Cyclic GMP‐AMP synthase (cGAS)* is a sensor of cytosolic double‐stranded DNA (ds‐DNA). ds‐DNA in the cytosol may occur from infection or mitochondrial damage. cGAS is activated by ds‐DNA binding to catalyze the cyclization of ATP and GTP to form a cyclic dinucleotide with mixed 2′,5′‐ and 3′,5′‐phosphodiester linkage (2′,3′‐cGAMP), which in turn activates stimulator of type 1 interferon genes (STING). Activated STING causes the activation of TBK1, which phosphorylates IRF3 allowing it to translocate to the nucleus where it triggers interferon‐inducible gene activation and interferon production. We report here the structure of cGAS with dinucleotides and small molecule inhibitors, and kinetic studies of the cGAS mechanism.

To study the β‐pseudo‐active form we obtained structures of an N‐terminal truncation of cGAS starting at residue 161 (cGAS161)22 in complex with five cyclic dinucleotides (2′,2′‐cGAMP, 2′,3′‐cGAMP, 3′,3′‐cGAMP, 3′,3′‐cdIMP and 3′,3′‐cdUMP), and the linear 2′,5′‐GpAp dinucleotide. There is no interaction between Asp227 and 3′,3′‐cdUMP or 2′,2′‐cGAMP; in these structures cGAS retains an inactive pose. 2′,2′‐cGAMP contains an amino group on its guanine base; however, 2′,2′‐cGAMP is considerably displaced from the active site compared with 2′,3′‐cGAMP or 3′,3′‐cGAMP with its amino group interacting with Asp319 (2.9 Å) instead of Asp227. Each compound binds to the same site formed between the side chains of Tyr436 and Arg376. This site is occupied by the adenine base in structures of ATP, 2′,2′‐cGAMP, 2′,3′‐cGAMP, or 3′,3′‐cGAMP, and is composed primarily of London dispersion interactions between the ring system of these binders with the phenyl ring of Try436. Most of these dinucleotides have affinities weaker than 500 μM (the top concentration tested).

>[2x]MGASKLRAVLEKLKLSRDDISTAAGMVKGVVDHLLLRLKCDSAFRGVGLLNTGSYYEHVKISAPNEFDVMFKLEVPRIQLEEYSNTRAYYFVKFKRNPKENPLSQFLEGEILSASKMLSKFRKIIKEEINDIKDTDVIMKRKRGGSPAVTLLISEKISVDITLALESKSSWPASTQEGLRIQNWLSAKVRKQLRLKPFYLVPKHAKEGNGFQEETWRLSFSHIEKEILNNHGKSKTCCENKEEKCCRKDCLKLMKYLLEQLKERFKDKKHLDKFSSYHVKTAFFHVCTQNPQDSQWDRKDLGLCFDNCVTYFLQCLRTEKLENYFIPEFNLFSSNLIDKRSKEFLTKQIEYERNNEFPVFDEF>[3x]NGPSPNLPPGFDFTDPAIYAERLPVAEFAELRSAAPIWWNGQDPGKGGGFHDGGFWAITKLNDVKEISRHSDVFSSYENGVIPRFKNDIAREDIEVQRFVMLNMDAPHHTRLRKIISRGFTPRAVGRLHDELQERAQKIAAEAAAAGSGDFVEQVSCELPLQAIAGLLGVPQEDRGKLFHWSNEMTGNEDPEYAHIDPKASSAEL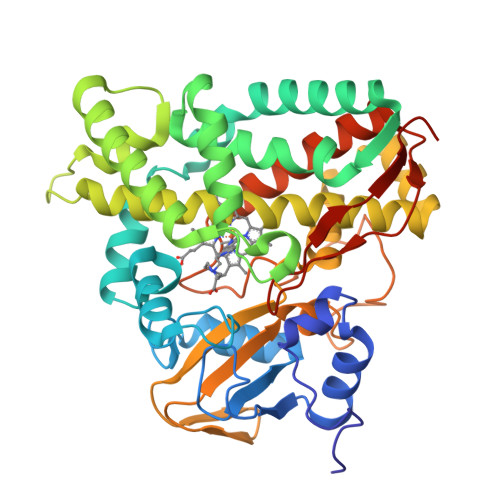IGYAMKMAEEKAKNPADDIVTQLIQADIDGEKLSDDEFGFFVVMLAVAGNETTRNSITQGMMAFAEHPDQWELYKKVRPETAADEIVRWATPVTAFQRTALRDYELSGVQIKKGQRVVMFYRSANFDEEVFQDPFTFNILRNPNPHVGFGGTGAHYCIGANLARMTINLIFNAVADHMPDLKPISAPERLRSGWLNGIKHWQVDYTGRCPVAH>STPGAQQVLFRTGIAAVNSTNHLRVYFQDVYGSIRESLYEGSWANGTEKNVIGNAKLGSPVAATSKELKHIRVYTLTEGNTLQEFAYDSGTGWYNGGLGGAKFQVAPYSCIAAVFLAGTDALQLRIYAQKPDNTIQEYMWNGDGWKEGTNLGGALPGTGIGATSFRYTDYNGPSIRIWFQTDDLKLVQRAYDPHKGWYPDLVTIFDRAPPRTAIAATSFGAGNSSIYMRIYFVNSDNTIWQVCWDHGKGYHDKGTITPVIQGSEVAIISWGSFANNGPDLRLYFQNGTYISAVSEWVWNRAHGSQLGRSALPPA[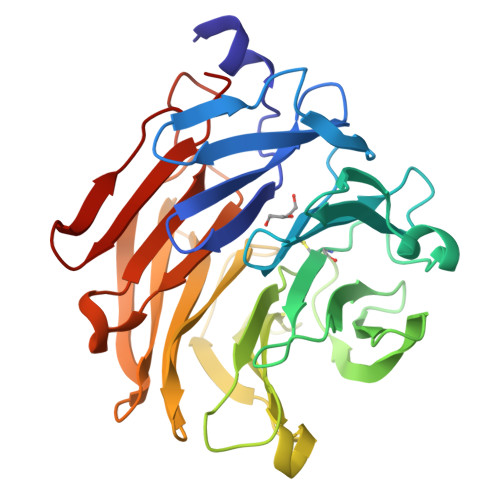4x]>MWFGEFGGQYVPETLVGPLKELEKAYKRFKDDEEFNRQLNYYLKTWAGRPTPLYYAKRLTEKIGGAKIYLKREDLVHGGAHKTNNAIGQAPLAKLMGKTRLIAETGAGQHGVATAMAGALLGMKVDIYMGAEDVERQKMNVFRMKLLGANVIPVNSGSRTAKDAINEALRDWEATFEYTHYLIGSVVGPHPYPTIVRDFQSVIGREAKAQILEAEGQLPDVIVACVGGGSNAMGIFYPFVNDKKVKLVGVEAGGKGLESGKHSASLNAGQVGVLHGMLSYFLQDEEGQIKPSHSIAPGLDYPGVGPEHAYLKKIQRAEYVTVTDEEALKAFHELSRTEGIIPALESAHAVAYAMKLAKEMSRDEIIIV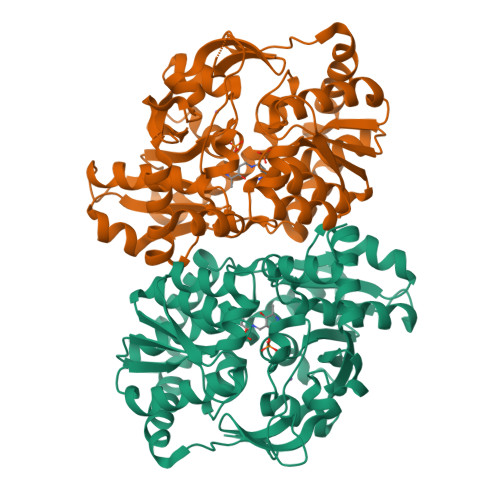NLSGRGDKDLDIVLKASGNV[4x]> GAMDP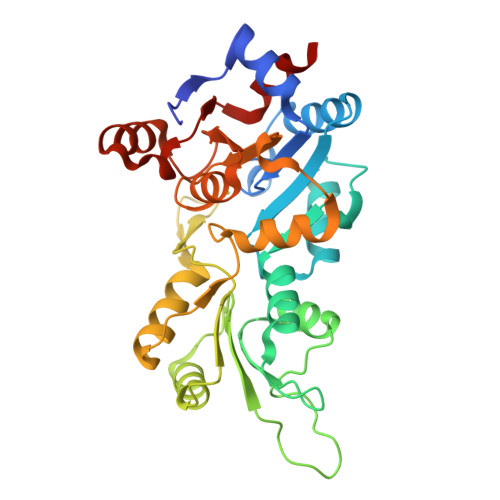MARCERLRGAALRDVLGRAQGVLFDCDGVLWNGERAVPGAPELLERLARAGKAALFVSNNSRRARPELALRFARLGFGGLRAEQLFSSALCAARLLRQRLPGPPDAPGAVFVLGGEGLRAELRAAGLRLAGDPSAGDGAAPRVRAVLVGYDEHFSFAKLREACAHLRDPECLLVATDRDPWHPLSDGSRTPGTGSLAAAVETASGRQALVVGKPSPYMFESITENFSIDPARTLMVGDRLETDILFGHRCGMTTVLTLTGVSRLEEAQAYLAAGQHDLVPHYYVESIADLTEGLED>MSLILSIVGTSDSGKTTLITRMMPILRERGLRVAVVKRHAHGDFEIDKEGKDSWKIYNSGADVVIASPVKLAFIRRVSEEEGNDLD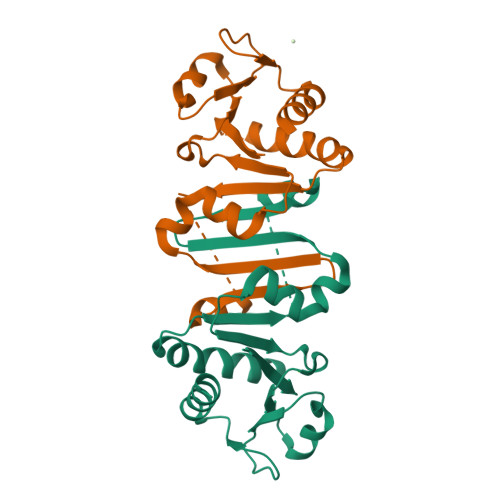WIYERYLSDYDLVITEGFSKAGKDRIVVVKKPEEVEHFRQGRILAVVCDERVDGHKWFRRDEVERIAEFILSLLREGGSHHHHHH[2x]>[2x]MAHHHHHHMPGSELISGGWFREENDQWPGQAMSLRVEKVLYDAPTKFQHLTIFESDPKGPWGTVMALDGCIQVTDYDEFVYHEVLGHTSLCSHPKPERVLIIGGGDGGVLREVLRHGTVEHCDLVDIDGEVMEQSKQHFPQISRSLADPRATVRVGDGLAFVRQTPDN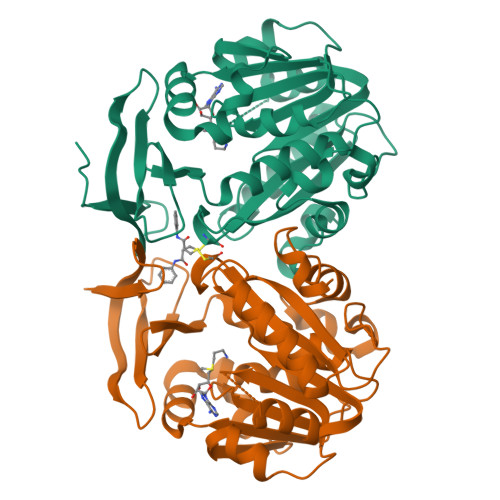TYDVVIIDTTDPAGPASKLFGEAFYKDVLRILKPDGICCNQGESIWLDLELIEKMSRFIRETGFASVQYALMHVPTYPCGSIGTLVCSKKAGVDVTKPLRPVEDMPFAKDLKYYDSEMHKASFALPRFARHINNSE> MVLGKPQTDPTLEWFLSHCHIHKYPSKSTLIHQGEKAETLYYIVKGSVAVLIKDEEGKEMILSYLNQGDFIGELGLFEEGQERSAWVRAKTACEVAEISYKKFRQLIQVNPDILMRLSAQM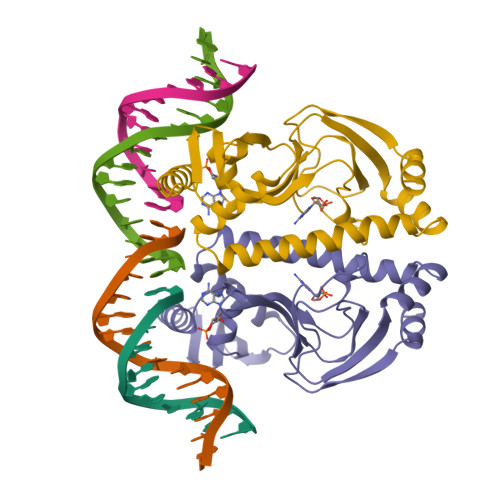ARRLQVTSEKVGNLAFLDVTGRIAQTLLNLAKQPDAMTHPDGMQIKITRQEIGQIVGCSRETVGRILKMLEDQNLISAHGKTIVVYGTR Integrins exist in a continuum of conformations between bent-closed non-ligand-bound (also termed inactive) and extended ligand-bound (also termed active) states. Glycosylation is required for integrin functions. Membrane distal N-glycosylation sites within the β-propeller domain of α5 and at the βI domain of β1 integrins are required for heterodimerization and efficient cell surface expression. For the conformationally switchable cell adhesion glycoprotein α5β1 integrin, we find that only the bent-closed state arranges N-glycans to nucleate the formation of up to tetrameric oligomers of the glycan-binding protein galectin-3.

To explore the molecular mechanism underlying the conformational state-specific dichotomic Gal3 oligomerization process, we set out to reveal the assembly state of Gal3 directly on inactive bent-closed α5β1 integrin via cryogenic electron microscopy (cryo-EM). We first vitrified peptidisc-embedded α5β1 integrin alone and refined the structure of the inactive bent-closed conformation to resolutions of 3.7 Å in the headpiece and 4.7 Å in the leg piece, respectively. A homology model of rat α5β1 integrin86 was fitted individually into the density maps of the headpiece (flexible fit) and leg piece (rigid-body fit). From the glycans of the α5 chain headpiece that point towards the additional cryo-EM density that we ascribed to Gal3, the one at position rN356 (hN307 in human α5) is a Gal3-binding competent complex-type glycan. Based on GlycoSHIELD modeling, it was indeed possible to position another Gal3 CRD for interaction with a galactose residue on the α5-rN356 (α5-hN307) glycan. With α5-rN918 (α5-hN867), α5-rN356 (α5-hN307) constitutes the core glycan pair, which is common to Gal3 dimers, trimers, and tetramers that all bridge the head and leg pieces of bent-closed α5β1 integrin (top, blue dashed line zoom). Our structural data pointed to the intriguing possibility that Gal3 oligomers might physically bridge membrane-proximal (leg piece) and distal (headpiece) parts of α5β1 integrin that face each other in the inactive bent-closed conformer. α5β1 integrin in its bent-closed state would thereby be stabilized by a Gal3-mediated clamping effect. Specifically, it appears that only on bent-closed α5β1 integrin N-glycans from head and leg pieces are arranged such that Gal3 oligomerization can be nucleated (left). In contrast, in extended ligand-bound α5β1 integrin, these glycans are too distant from each other to enable such oligomerization (right). We think that our structural determination of the first example of Gal3 nucleation on spatially arranged N-glycans in the inactive bent-closed state of α5β1 integrin provides a guide for the N-glycan arrangement pattern needed to nucleate Gal3 oligomers and ultimately for predicting glycoproteins that are capable of doing so.

> MPPRQPTRRPGGGPSRELGKLLPALSHSPLGGLGSGSGSVAPGQGRTGAMGSWTPRSPRSPLHAVLLRWGPRRLPPLLPLLLLLWPPPLQVGGFNLDAEAPAVLSGPPGSLFGFSVEFYRPGRDGVSVLVGAPKANTSQPGVLQGGAVYVCPWGTSPIQCSTIQFDSKGSRILESSLYSEEPVEYKSLQWFGATVRAHGSSILACAPLYSWRTEKDPQNDPVGTCYLSTENFTRILEYAPCRSDFGSAAGQGYCQGGFSAEFTKTGRVVLGGPGSYFWQGQILSATQEQISESYYPQYLINPVQGQLQTRQASSVYDDSYLGYSVAVGEFSGDDTEDFVAGVPKGNLTYGYVTVLNGSDIHSLYNVSGEQMASYFGYAVAATDTNGDGLDDLLVGAPLLMERTADGRPQEVGRVYIYLQHPEGIEPTPSLTLTGQDEFGRFGSSLTPLGDLDQDGYNDVAIGAPFGGEAQQGVVFIFPGGPGGLNTKPSQVLQPLWAAGHTPDFFGSALRGGRDLDGNGYPDLIVGSFGVDKALVYRGRPIISASASLTIFPSMFNPEERSCSLEGNPVSCINLSFCLNASGKHVPNSIGFEVELQLDWQKQKGGVRRALFLASKQATLTQTLLIQNGAREDCREMKIYLRNESEFRDKLSPIHIALNFSLDPKAPMDSHGLRPVLHYQSKSRIEDKAQILLDCGEDNICVPDLQLAVYGEKKHVYLGDKNALNLTFLAQNLGEGGAYEAELRVTAPLEAEYSGLVRHPGNFSSLSCDYFAVNQSRQLVCDLGNPMKAGTSIWGGLRFTVPHLQDTKKTIQFDFQILSKNLNNSQSNMVSFPLSVEAQAQVSLNGVSKPEAVIFPVSDWNPQDQPQKEGDLGPAVHHVYELINQGPSSISQGVLEISCPQALEGQQLLYVTKVTGLNNCTSNYTPNSQGLELDPEVSPHHLQRREAPGRSSTTSGTQVLKCPEAKCFRLRCEFGPLHRQESRSLQLHFRVWAKTFLQQEYQPFSLQCEALYEALKMPYQILPRQLPQKKLQVATAVQWTKAEGSNGVPLWIIILAILFGLLLLGLLIYVLYKLGFFKRSLPYGTAMEKAQLKPPATSDA;> MNLQLVFWIGLISLICSVFGQTDKNRCLKANAKSCGECIQAGPNCGWCTNTTFLQEGMPTSARCDDLEALKKKGCHPSDIENPRGSQTIKKNKNVTNRSKGMAEKLRPEDITQIQPQQLLLKLRSGEPQKFTLKFKRAEDYPIDLYYLMDLSYSMKDDLENVKSLGTDLMNEMRRITSDFRIGFGSFVEKTVMPYISTTPAKLRNPCTSEQNCTSPFSYKNVLSLTDRGEFFNELVGQQRISGNLDSPEGGFDAIMQVAVCGSLIGWRNVTRLLVFSTDAGFHFAGDGKLGGIVLPNDGQCHLENNVYTMSHYYDYPSAIHLVQKLSENNIQTIFAVTEEFQPVYKELKNLIPKSAVGTLSGNSSNVIQLIIDAYNSLSSEVILENSKLPDGVTINYKSYCKNGVNGTGENGRKCSNISIGDEVQFEISITANKCPNKESENQLKLNPLGFTEEVEVVLQFICKCNCQSHGIPASPKCHEGNGTFECGACRCNEGRVGRHCECSTDEVNSEDMDAYCRKENSSEICSNNGECVCGQCVCRKRENTNEIYSGKFCECDNFNCDRSNGLICGGNGVCRCRVCECYPNYTGSACDCSLDTVPCVATNGQICNGRGICECGACKCTDPKFQGPTCETCQTCLGVCAEHKECVQCRAFNKGEKKDTCAQECSHFNLTKVESREKLPQPVQVDPVTHCKEKDIDDCWFYFTYSVNSKGEAHVHVVETPDCPTGPDIIPIVAGVVAGIVLIGLALLLIWKLLMIIHDRREFAKFEKEKMNAKWDTGENPIYKSAVTTVVNPKYEGK>SNAMTERGLLIVLSGPSGVGKGTVREAVFKDPETSFDYSISMTTRLPREGEQDGVDYYFRSREVFEQAIKDGKMLEYAEYVGNYYGTPLEYVEEKLAAGVDIFLEIEVQGAMQVRKAMPEGIFIFLTPPDLSELKNRIIGRGTESMEVVEERMETAKKEIEMMASYDYAVVNDVVANAVQKIKGIVETEHLKTERVIH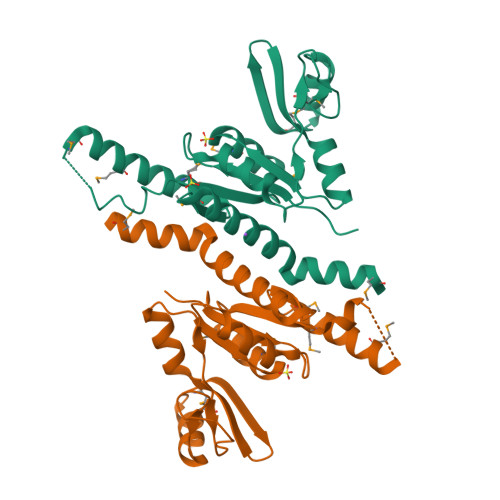RYKKMLEGLQ[2x]> QDPIKFTTGSATPASY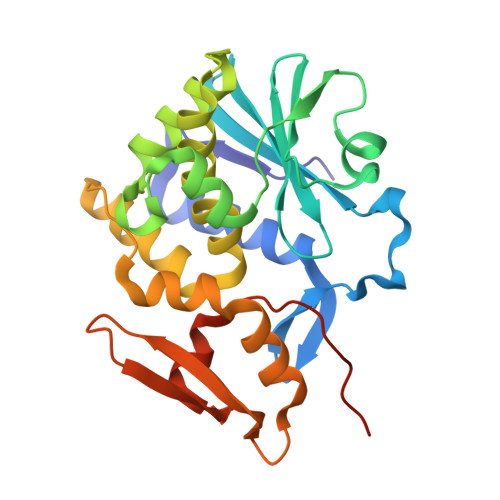NQFIDALRERLTGGLIYGIPVLRDPSTVEKPNQYVTVELSYSDTVSIQLGIDLTNAYVVAYRAGSESFFFRNAPASASTYLFTGTQQYSLPFDGNYDDLEKWAHQSRQRISLGLEALRQGIKFLRSGASDDEEIARTLIVIIQMVAEAARFRYVSKLVVISLSNRAAFQPDPSMLSLENTWEPLSRAVQHTVQDTFPQNVTLINVRQERVVVSSLSHPSVSALALMLFVCNPLNATQSPLLI2-AMINO-4-TRIFLUOROMETHYLSULFANYL-BUTYRIC ACID | C5 H8 F3 N O2 S | 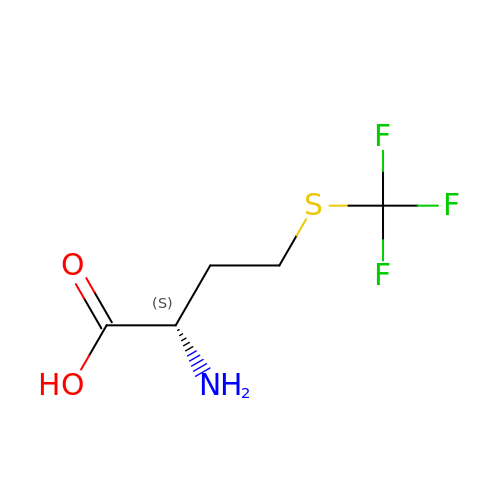YLJLTSVBCXYTQK-VKHMYHEASA-N>[8x]MASSHHHHHHSSGLVPRGSSMG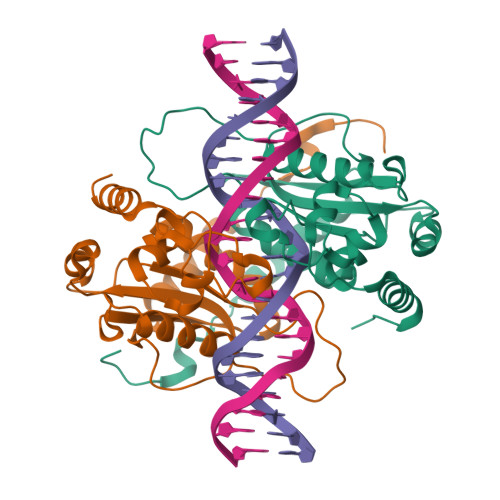HNKKFDRSEHVYRNDSFLELIKDAVRFFSGTPVHSLPPPERFQGAGVYALYYTGHYSLYDEYSRINRKAYNLPIYVGKAVPAGWRQSRISDHETRAGSELSNRIREHGRNIAKTSNLDLCDFSCRFVIFEATGSDMISTVQAALIKIYKPLWNTVVDGFGNHTPGAGRFAQAKSDWDVIHPGREWAEKCTGVHSEPYFIEERIKQYFSKSNFT> GAGCAGCCTGT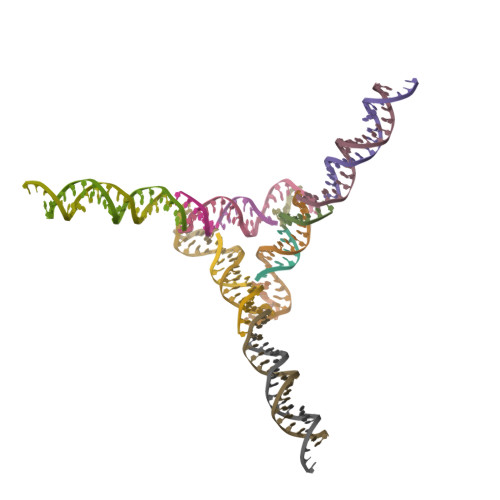ACGGACATCA;> CCGTACA;> TCTGATGT;> GGCTGC;> GATGCTGACGTAGTAGCAGAG;> TCCTCTGCTACTACGTCAGCA>[3x]GSHMFKVKKLSDKAIIPQRGSKGAAGYDLSSAHELVVPAHGKALAMTDLQIAIPDGTYGRIAPRSGLAWKNFIDCGAGVIDSDYRGNVGVVLFNHSDVDFKVAVGDRVAQLIFE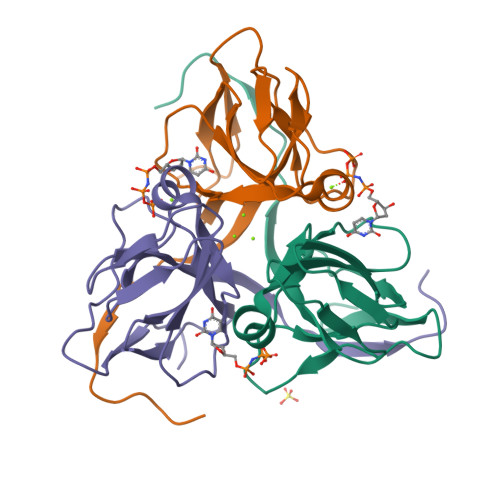RIVTPEPLEVDEIDETQRGAGGFGSTGVKVQN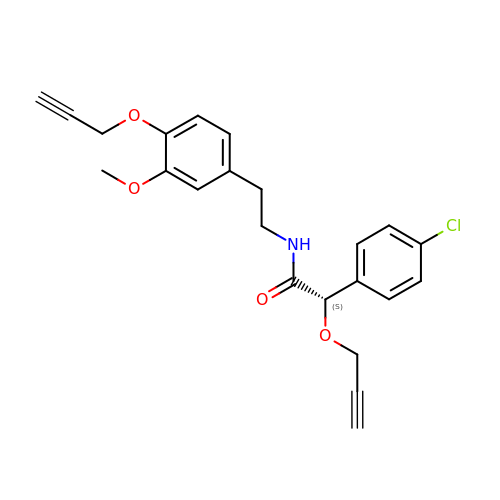(2S)-2-(4-chlorophenyl)-N-{2-[3-methoxy-4-(prop-2-yn-1-yloxy)phenyl]ethyl}-2-(prop-2-yn-1-yloxy)ethanamide | C23 H22 Cl N O4 | KWLVWJPJKJMCSH-QFIPXVFZSA-N~{N}-[(2~{S},3~{R},4~{R},5~{S},6~{R})-6-[[(4-cyanophenyl)sulfonylamino]methyl]-2,4,5-tris(oxidanyl)oxan-3-yl]-3-phenyl-benzamide 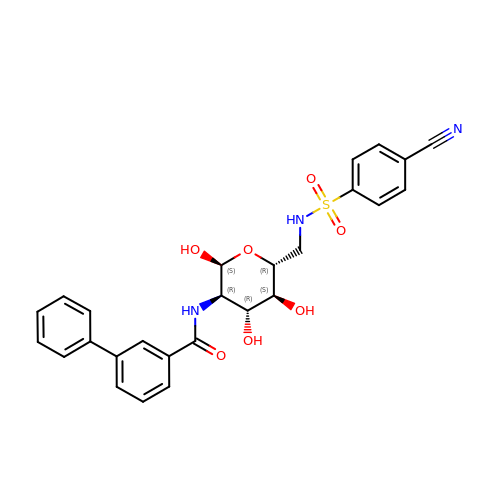| C26 H25 N3 O7 S | MPZFVCYRXPGUGA-YLLXKFEGSA-N>SNAMKD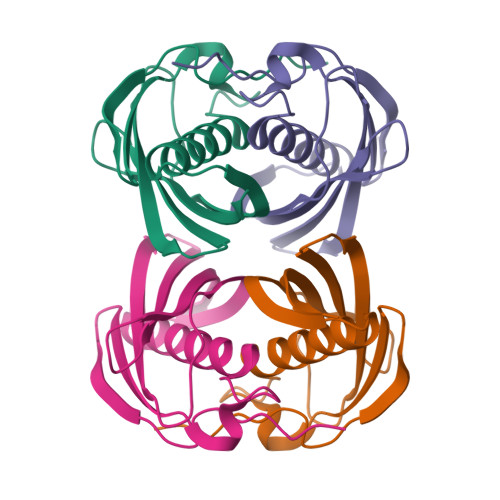FHFDAISAFENYEIEKMRDGHVVVTTKVVNSSLNYYGNAHGGYLFTLCDQISGLVVISLGLDGVTLQSSINYLKAGKLDDVLTIKGECVHQGRTTCVMDVDITNQEGRNVCKATFTMFVTGQRSEERRVRI[2x]> HRK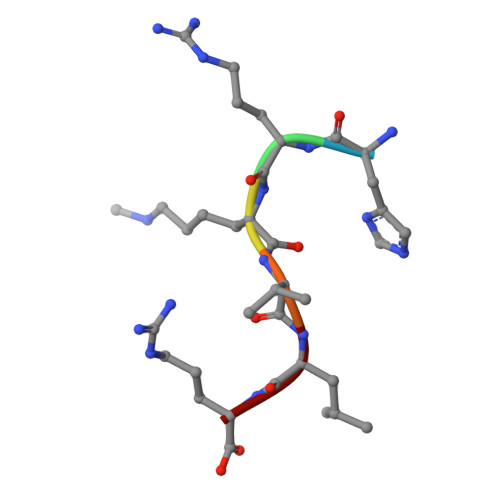VLR N-ACETYL-L-ILE-L-TYR-(R)-1-AMINO-2-(4-HYDROXYPHENYL)ETHYLPHOSPHONIC ACID | C25 H34 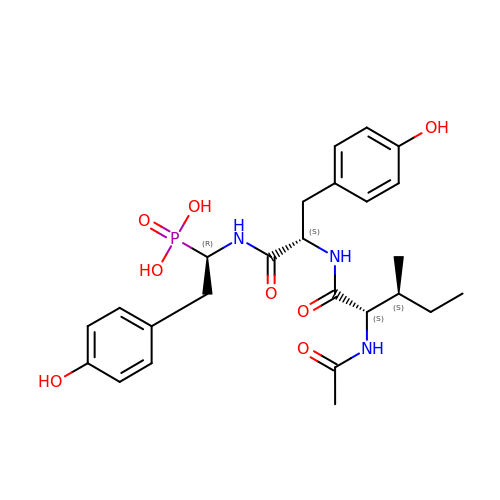N3 O8 P | ZFRNBYWFOLDQKG-FDMHNHSTSA-N1-[5-(4-amino-7-methyl-7H-pyrrolo[2,3-d]pyrimidin-5-yl)-4-fluoro-1H-indol-1-yl]-2-(6-methylpyridin-2-yl)ethanone | C23 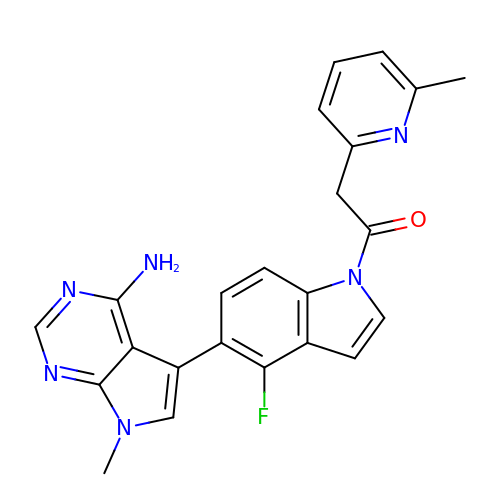H19 F N6 O | YGEJQNSKXJFIJF-UHFFFAOYSA-N> MKTVTVKNLIIGEGMPKIIVSLMGRDINSVKAEALAYREATFDILEWRVDHFMDIAST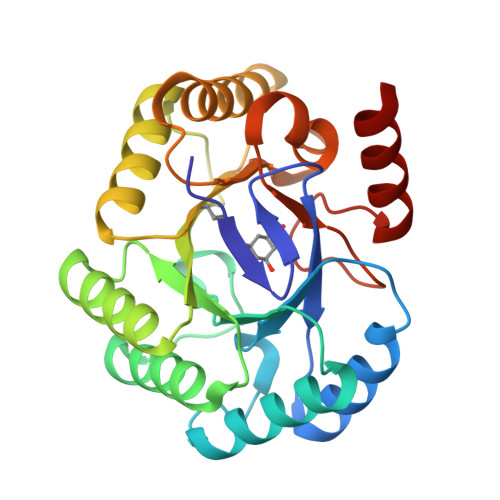QSVLTAARVIRDAMPDIPLLFTFRSAKEGGEQTITTQHYLTLNRAAIDSGLVDMIDLELFTGDADVKATVDYAHAHNVYVVMSNHDFHQTPSAEEMVLRLRKMQALGADIPKIAVMPQSKHDVLTLLTATLEMQQHYADRPVITMSMAKEGVISRLAGEVFGSAATFGAVKQASAPGQIAVNDLRSVLMILHNA> ANGTSSAFTQVDNFSHFYDRGNHLVNGKPSFTVDQAADQLTRSGASWYDLNGDGVINLSYTFLTSPPPGYASRGLGTFSSFSGLQKEQAKLSLESWADVAKVTFTEGPAARGDDGHMTFANFSASNGGAAFAYLPNSSRKGESWYLINKDYDVNKTPGEGNYGRQTLTHEIGHTLGLSHPGDYNAGNGNPSYRDAVYGEDTRAYSVMSYWSEKNTGQVFTKTGEGAYASAPLLDDIAAVQKLYGANMETRAGDTVYGFNSTADRDYYSATSATDKLIFSVWDGGGNDTLDFSGFSQNQKINLAAGSFSDVGGMTGNVSIAQGVTIENAIGGSGNDLLLGNAASNILKGGAGNDIIYGGGGADKLWGGSGSDTFVYREVSDSTPKAADTLMDFQTGLDKIDLTGITHLSGLNFVNAFTGQAGDAVVSYNQASNAGSLQVDFSGHGVADFLITTVGQVAT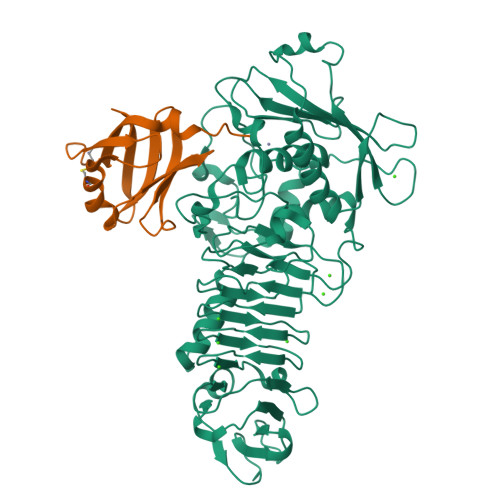YDIVA;> SLMLLSPAQVAGSWTFYVQGAEQDACTVTLKKDRTFSAQVSCLQAWLGRTPTTWSPTPDGLLLIGKDGSQSLFLELREAGRYEGSVEGSKTLVMQRA>[4x]MSAKAISEQTGKELLYKFICTTSAIQNRFKYARVTPDTDWARLLQDHPWLLSQNLVVKPDQLIKRRGKLGLVGVNLTLDGVKSWLKPRLGQEATVGKATGFLKNFLIEPFVPHSQAEEFYVCIYATREGDYVLF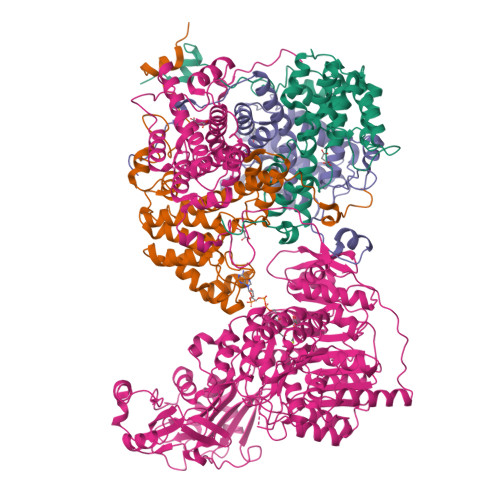HHEGGVDVGDVDAKAQKLLVGVDEKLNPEDIKKHLLVHAPEDKKEILASFISGLFNFYEDLYFTYLEINPLVVTKDGVYVLDLAAKVDATADYICKVKWGDIEFPPPFGREAYPEEAYIADLDAKSGASLKLTLLNPKGRIWTMVAGGGASVVYSDTICDLGGVNELANYGEYSGAPSEQQTYDYAKTILSLMTREKHPDGKILIIGGSIANFTNVAATFKGIVRAIRDYQGPLKEHEVTIFVRRGGPNYQEGLRVMGEVGKTTGIPIHVFGTETHMTAIVGMALGHRPIPNQPPTAAHTANFLLNASGSTSTPAPSRTASFSESRADEVAPAKKAKPAMPQDSVPSPRSLQGKSTTLFSRHTKAIVWGMQTRAVQGMLDFDYVCSRDEPSVAAMVYPFTGDHKQKFYWGHKEILIPVFKNMADAMRKHPEVDVLINFASLRSAYDSTMETMNYAQIRTIAIIAEGIPEALTRKLIKKADQKGVTIIGPATVGGIKPGCFKIGNTGGMLDNILASKLYRPGSVAYVSRSGGMSNELNNIISRTTDGVYEGVAIGGDRYPGSTFMDHVLRYQDTPGVKMIVVLGEIGGTEEYKICRGIKEGRLTKPIVCWCIGTCATMFSSEVQFGHAGACANQASETAVAKNQALKEAGVFVPRSFDELGEIIQSVYEDLVANGVIVPAQEVPPPTVPMDYSWARELGLIRKPASFMTSICDERGQELIYAGMPITEVFKEEMGIGGVLGLLWFQKRLPKYSCQFIEMCLMVTADHGPAVSGAHNTIICARAGKDLVSSLTSGLLTIGDRFGGALDAAAKMFSKAFDSGIIPMEFVNKMKKEGKLIMGIGHRVKSINNPDMRVQILKDYVRQHFPATPLLDYALEVEKITTSKKPNLILNVDGLIGVAFVDMLRNCGSFTREEADEYIDIGALNGIFVLGRSMGFIGHYLDQKRLKQGLYRHPWDDISYVLPEHMSM4-hydroxy-6-methyl-2H-1-benzopyran-2-one 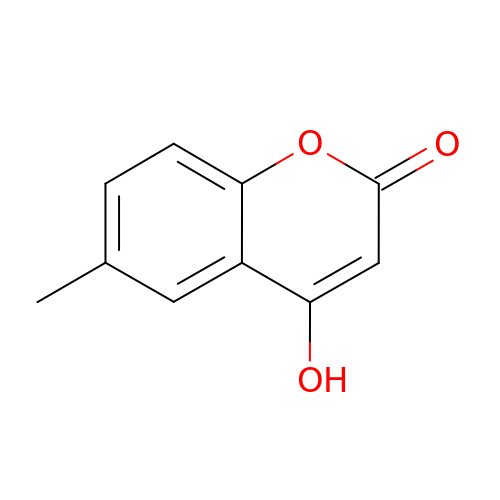| C10 H8 O3 | WIRGBZBGYNIZIB-UHFFFAOYSA-N> MSVKRRTFLQGAAGAIGLAMAQGALSKIVYAQGAAGTLRVAIAKPAGNLDPQSHYAIWAIQDLMFEPLVKYGKGGQIEPCLATDWKIEDGGKTLHLTLREGVKFQDGTKFDAAACKWNLERWMGIDQFSWMNCSKHFQSLEVVDDYHITVHFKEPVLALMQELSYTRPTRFLSPKSVDADGKFKEPVGTGPWVQISADDTQSVFEHYDGYWGDKPTYERLEAKVIPDARSRVAALRAG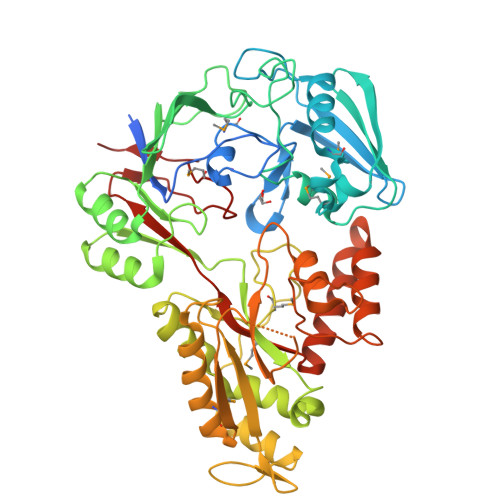EIDLVGGFWIAPLTPEEGKQLEAAGFNVVVDPGNVTLVMAFNPDRAEPLKDPQVRKAVSIGIDRAAISKVLYHGYAKPAGNMFSAALPYAGKQFDAPVRDAAAASALLEKAGWTGSPIRSKDGKPLTLELVVSPDAVPGSRVIAEVIQSEMKEVGIDLVIRSVDHASKHTDMLEQKYDLGFFLTYGAPYDPFGSLVALCLSTFKNDVEGKLVTDPVNLDPLINAATAATGDQIEPTIQKVYDWLRDNDAIAPLVYVPSIWAHSKRVQGFTSPVTEYDMPYENIVLAE> TKQ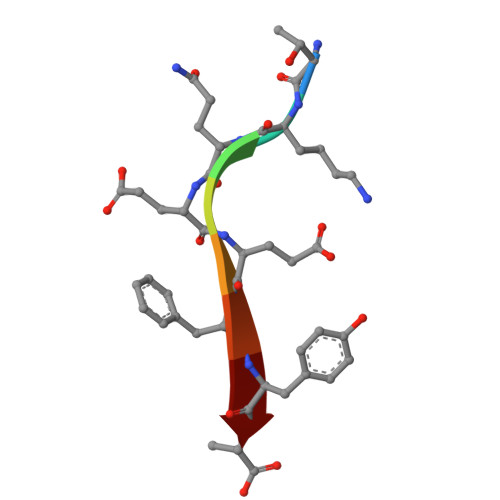EEFYA>[2x]GSSHHHHHHMGNVFDYEDIQLIPAKCIVNSRSECDTTVTLGKHKFKLPVVPANMQTIIDERIATYLAENNYFYIMHRFQPEKRISFIRDMQSRGLIASISVGVKEDEYEFVQQLAAEHLTPEYITI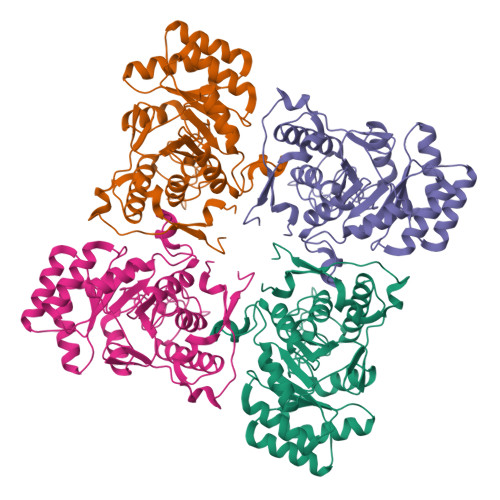DIAHGHSNAVINMIQHIKKHLPESFVIAGNVGTPEAVRELENAGADATKVGIGPGKVCITKIKTGFGTGGWQLAALRWCAKAASKPIIADGGIRTNGDVAKSIRFGATMVMIGSLFAGHEESPGETIEKDGKLYKEYFGSASEFQKGEKKNVEGKKMFVEHKGSLEDTLIEMEQDLQSSISYAGGTKLDSIRTVDYVVVKNSIFNGDKVY>[2x]SNAMQLTSQAFSYGRPIPKKYSCQGVGISPPLSFSDVPREAKSLVLIVEDPDVPPSVREDG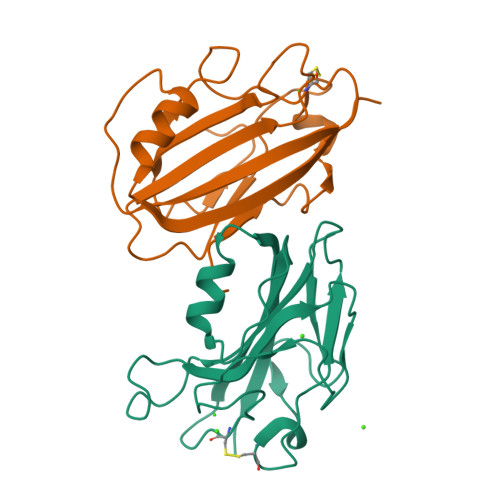LWIHWIVYNLSPVVSNLAEGAQIFAVQGLNTAGEIGYCPPCPPDAKHRYYFYAYALDVVLSDEEGVTKEQLLEAMDGHIIATAELMGTYEKD> MSILVNKNTKVIVQGFTGKEATFHAEQCMAYGTNIVGGITPHKGGQTHLGKPVFDTVADAVKATKADVSLIFVPAFAVGDSVIEAADAGIKL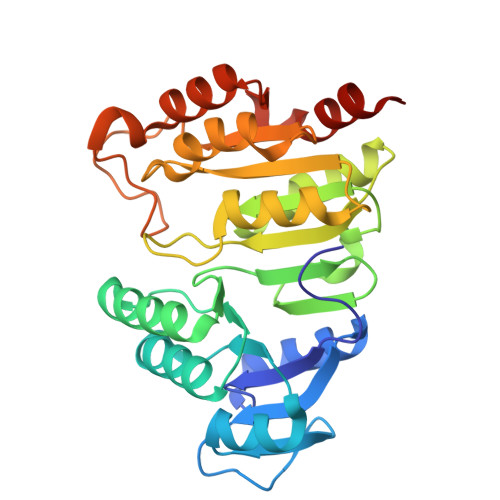AVVITEHTPVKDMMFAKQYANKKGMKIIGPNCPGIITSEECKLGIMPGFIFKKGCVGLISKSGTLTYEAANQVVQGGYGISTAVGIGGDPIIGLAYKELLSEFQKDDETKAIVMIGEIGGSLEVEAAKFIKENISKPVVAFIAGATAPKGKRMGHAGAIVGSADESAAAKKEALKSYGIHVVDSPALIGEEIQKILGENLYFQ[[(3R,4R,5S,6R)-3-(BUTANOYLAMINO)-4,5-DIHYDROXY-6-(HYDROXYMETHYL)OXAN-2-YLIDENE]AMINO] N-PHENYLCARBAMATE | C17 H23 N3 O7 | 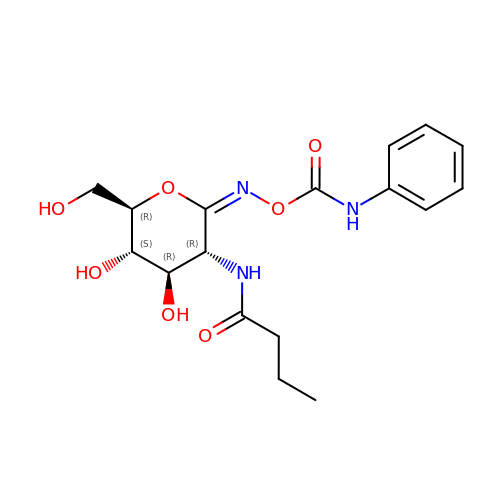ITVRELFVFCOUMV-ZVZWZHPPSA-N>INFDQIFEGAIEPGKEPKRLFKEVYEGAITATSYAEILLSRAIEKYGPDHPVGYPDTAYFLPVIRAFSGEEVRTLKDMVPILNRMRAQIKSELTFENARLAGEATWYAAEIIEALRYLKHTPENPIVVPPWTGFIGDPVVRQYGIKMVDWTIPGEAIIIGRAKDSKAAKKIVDDLMGKGLMLFLCDEIIEQLLEENVKLGVDYIAYPLGNFTQVVHAANYALRAGLMFGGIAPGLRDAHRDYQRRRVLAFVLYLGEHDMVKTAAAMGAIFTGFPVITDQPLPEDKQIKDWFISEPDYDKIVQTALEVRGIKITSIDIDLPINFGPAFEGESIRKGDMHVEFGGGKTPSFELVRMVGPDEIEDGKVEVIGPDIDSVEPGGRLPIGIVVDIYGRKMQEDFEPVLERRIHYFTNYGEGFWHTAQRDLTWVRISKEAFAKGARLKHLGQLLYAKFKQEFPSIVDRVQVTIYTDEQKVLELREIARKKYAERDARLRELSDEAVDTYYSCLLCQSFAPTHVCIVSPERVGLCGAISWLDAKAAYEINPNGPNQPIPKEGLIDPVKGQWESFNEYIYKNSQRTIERMNLYTIMEYPMTSCGCFEAIMAYLPELNGFMIVNREHSGMTPIGMTFSTLAGMVGGGTQTPGFMGIGKSYIGSRKFVKADGGLARVVWMPKDLKEQLRSIIEERAEEEGLGRDFIDKIADETVGTTVDEVLPFLEEKGHPALSMEPLLRSHH[3x]

CO-dehydrogenase (CODH)–acetyl-coenzyme A synthase (ACS) is an enzyme complex in the reductive acetyl-coenzyme A (acetyl-CoA) pathway that reduces two molecules of CO2 to acetyl-CoA. Finally, the two branches merge through the action of ACS, which catalyses the condensation of CO, the CH3 moiety and CoA to yield acetyl-CoA. ACS binds substrates at cluster A. Cluster A is a [4Fe4S] cluster connected by a cysteine to two Ni atoms that are bridged by two further cysteines. The Ni ion proximal (proximal Ni, Nip) to the [4Fe4S] cluster is the site of catalysis, while the distal Ni ion most probably plays a structural role as its oxidation state is unchanged during catalysis.

Three main species were found in untreated as-isolated CODH–ACS that are denoted wobbly, half-closed and triangle based on the arrangement of the ACS domain. On the wobbly side, the N-terminal ACS domain resembles that of the crystal structure of the open state. The triangle state is an artefact due to the binding of the 6xHis tag to cluster A (Supplementary Discussion). The triangle state was not considered for the ACS conformations as it is not physiologically relevant and is probably an artefact of the interaction of the ACS-6xHis tag with the Nip. The triangle state was not found in the reduced state, which could be due to the reduced affinity of Ni ions to histidine after reduction.>[2x]SNAMALKKPGSLTIAGSGIASIGHITLETLALIKEADKIFYAVTDPATECYIQENSRGDHFDLTTFYDTNKKRYESYVQMSEVMLRDVRAGRNVLGIFYGHPGVFVAPSHRAIAIAREEGFQAKMLPGISAEDYMFADLGFDPSTYGCMTQEATELLVRNKKLDPSIHNIIWQVGSVGVDTMVFDN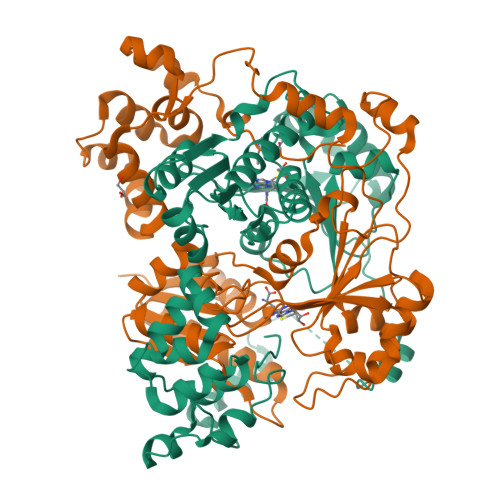GKFHLLVERLEKDFGLDHKIQHYIGAILPQSVTVKDTFAIRDLRKEEVLKQFTTTSTFYVPPRTPAPIDPKAVQALGLPATVTKGAQDWTGFQSVSPAYGPDEMRAVAALDSFVPSQEKAVVHASRAMQSLMVDLALRPALLEQYKADPVAFANTRNGLTAQEKFALGLKKPGPIFVVMRQLPSAIASGQEPSQEEIARADDATAFIIIYIVQG;>SNAMALKKPGSLTIAGSGIASIGHITLETLALIKEADKIFYAVTDPATECYIQENSRGDHFDLTTFYDTNKKRYESYVQMSEVMLRDVRAGRNVLGIFYGHPGVFVAPSHRAIAIAREEGFQAKMLPGISAEDYMFADLGFDPSTYGCMTQEATELLVRNKKLDPSIHNIIWQVGSVGVDTMVFDNGKFHLLVERLEKDFGLDHKIQHYIGAILPQSVTVKDTFAIRDLRKEEVLKQFTTTSTFYVPPRTPAPIDPKAVQALGLPATVTKGAQDWTGFQSVSPAYGPDEMRAVAALDSFVPSQEKAVVHASRAMQSLMVDLALRPALLEQYKADPVAFANTRNGLTAQEKFALGLKKPGPIFVVMRQLPSAIASGQEPSQEEIARADDATAFIIIXIVQG[2x]>[2x]ASMTGNECPELQPPVHGKIEPSQAKYFFKDQVLVSCDTGYKVLKDNVEMDTFQIECLKDGTWSNKIPTCKIVDCRAPGELEHGLITFSTRNNLTTYKSEIKYSCQEPYYKMLNNNTGIYTCSAQGVWMNKVLGRSLPTCLPVCGLPKFSRKLMAR;>[2x]IFNGRPAQKGTTPWIAMLSHLNGQPFCGGSLLGSS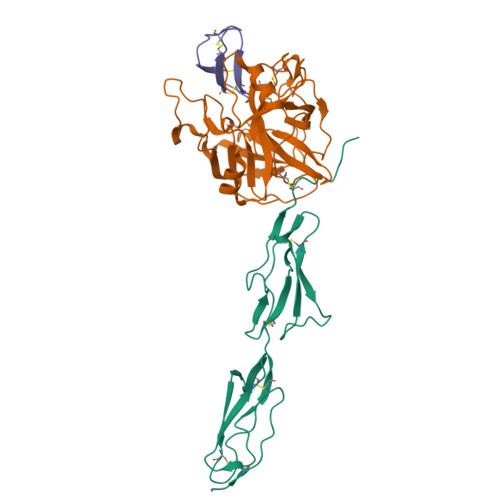WIVTAAHCLHQSLDPKDPTLRDSDLLSPSDFKIILGKHWRLRSDENEQHLGVKHTTLHPQYDPNTFENDVALVELLESPVLNAFVMPICLPEGPQQEGAMVIVSGWGKQFLQRFPETLMEIEIPIVDHSTCQKAYAPLKKKVTRDMICAGEKEGGKDACAGDSGGPMVTLNRERGQWYLVGTVSWGDDCGKKDRYGVYSYIHHNKDWIQRVTGVRN;>[2x]GSGEVTCEPGTTFKDKCNTCRCGSDGKSAFCTRKLCYQ>[2x]MPPETATNPKDARHDGWQTLKRFLPYLWPADNAVLRRRVVGAILMVLLGKATTLALPFAYKKAVDAMTLGGGAQPALTVALAFVLAYALGRF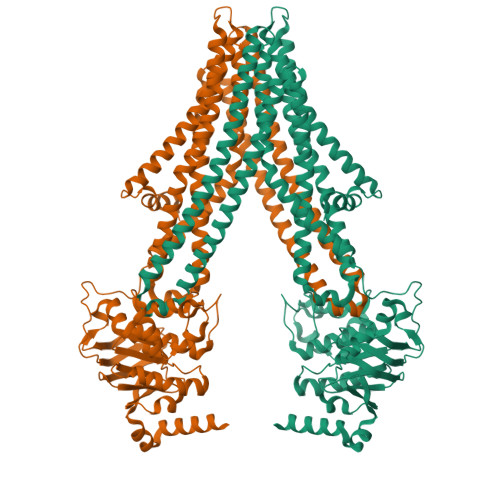SGVLFDNLRNIVFERVGQDATRHLAENVFARLHKLSLRFHLARRTGEVTKVIERGTKSIDTMLYFLLFNIAPTVIELTAVIVIFWLNFGLGLVTATILAVIAYVWTTRTITEWRTHLREKMNRLDGQALARAVDSLLNYETVKYFGAESREEARYASAARAYADAAVKSENSLGLLNIAQALIVNLLMAGAMAWTVYGWSQGKLTVGDLVFVNTYLTQLFRPLDMLGMVYRTIRQGLIDMAEMFRLIDTHIEVADVPNAPALVVNRPSVTFDNVVFGYDRDREILHGLSFEVAAGSRVAIVGPSGAGKSTIARLLFRFYDPWEGRILIDGQDIAHVTQTSLRAALGIVPQDSVLFNDTIGYNIAYGRDGASRAEVDAAAKGAAIADFIARLPQGYDTEVGERGLKLSGGEKQRVAIARTLVKNPPILLFDEATSALDTRTEQDILSTMRAVASHRTTISIAHRLSTIADSDTILVLDQGRLAEQGSHLDLLRRDGLYAEMWARQAAESAEVSEAAEHHHHHH>MSVMFDPQSYPYPSRRNVVYAKNGMVATSQPLAAQAGLDILKAGGNAIDAAIATATALTVLEPTSNGIGSDAFALVWTKGKLHGLNGSGRAPMSLTMEAVKAKGYEQELPPYGVIPVTVPGAPGAWAELAKMYGNLPLAASLAPAIRYAEEGYPVTPTLAKYWKAAYDRVKTEWTDDVYQPWFDTFAPKGRAPRVGEVWRSQGHADTLRSIAESNGESFYRGELADQIHAFFDKHGGYLTKEDLACYRPEWVEPISIDYRGYRVWEIPPNGQGLVALEALNIVKGFEFYHKDTVDTYHKQIEAMKLAFVDGMKYVTEPSDMSVSVEQLLSDEYATERRKEIGEQALTPEPGTPPRGGTVYLATADGDGNMVSFIQSNYMGFGSGVVVPGTGIAMQNRGHNFSLDPNHDNALKPGKRTYHTIIPGFLTKNDQPIGPFGVMGGFMQPQGHMQVMMNTIDFGLNPQAALDAPRWQWTNGKQVQVEPTFPVDIAQALVRRGHKIQVVLDEGAFGRGQIIWRDPTTGVLAGGTEPRTDGQVAAW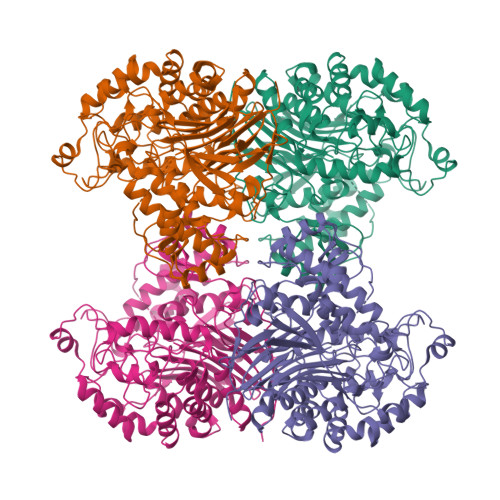EGHHHHHH[4x]>[4x]MPPSLRKAVAAAIGGGAIA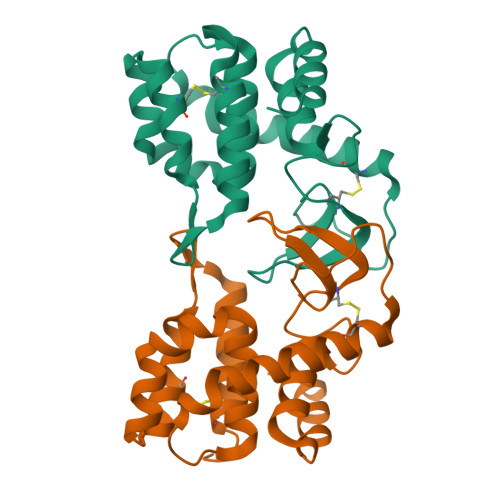IASVLITGPSGNDGLEGVSYIPYKDIVGVWTVCHGHTGKDIMLGKTYTKAECKALLNKDLATVARQINPYIKVDIPETMRGALYSFVYNVGAGNFRTSTLLRKINQGDIKGACDQLRRWTYAGGKQWKGLMTRREIEREICLWGQQ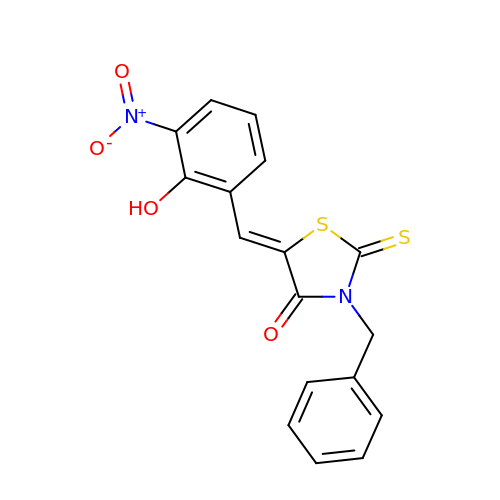(Z)-3-BENZYL-5-(2-HYDROXY-3-NITROBENZYLIDENE)-2-THIOXOTHIAZOLIDIN-4-ONE | C17 H12 N2 O4 S2 | ZTWBCEZQPRYIGY-ZROIWOOFSA-N2-methoxy-4-[6-(propan-2-ylamino)imidazo[1,2-b]pyridazin-3-yl]benzamide | C17 H19 N5 O2 | 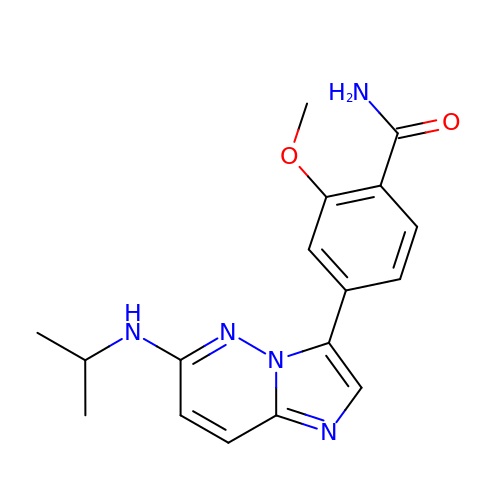IBZJJCFFBCEGPS-UHFFFAOYSA-N>[2x]GSFKFTAQQHVYDINGVKVGGQPGEYPTVLIGSIFYRGHKIVSDGQKGIFDKDAAKALLDQEAELSAETGNPFIIDVLGESVEALTKYVEFILENTTAPFLLDSISPDVRVGALKNLGKDPEIQKRLIYNSIEEHYTEEELAAIKEAGLKTAVILAFSKKALKPNARIDLLQGKDDKEGLIAAAKRAGIEQFLVDPGVLDVASNSWTTEAINVVKEQFGYPGGCAPSAAVYLWKKMRSKGTPFFEVAGAAVFTYPITQGADFILYGPMMNAPWVYRAIATTDAMIAYNNKLTGVKMGTTEHPLLKIF

During energy production in Desulfitobacterium hafniense, MtgA catalyzes the methyl transfer from methylcobalamin (Cbl‐CH3) to THF in the catabolism of glycine betaine (GB). Despite its lack of sequence identity with known structures, we could show that MtgA forms a homodimeric complex of two TIM barrels. The topology of each subunit is characterized by a funnel of eight parallel β‐sheets connected by α‐helices on the outside that form a complex of two perpendicularly oriented TIM barrels. The active‐site cavity is located inside the hydrophilic core of each barrel.

Apart from snapshots of individual reaction steps of MtgA, structure‐based mutagenesis combined with enzymatic activity assays allowed a mechanistic description of the methyl transfer between Cbl‐CH3 and THF.> GSKKLINDVQDVLDEQLAGLAKAHPSLTLHQDPVYVTRADAPVAGKVALLSGGGSGHEPMHCGYIGQGMLSGACPGEIFTSPTPDKIFECAMQVDGGEGVLLIIKNYTGDILNFETATELLHDSGVKVTTVVIDDDVAVK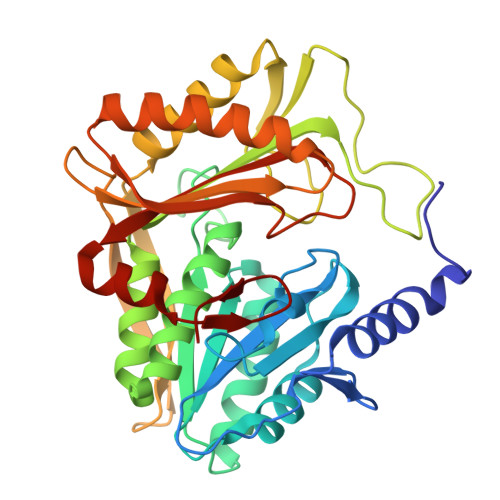DSLYTAGRRGVANTVLIEKLVGAAAERGDSLDACAELGRKLNNQGHSIGIALGACTVPAAGKPSFTLADNEMEFGVGIHGEPGIDRRPFSSLDQTVDEMFDTLLVNGSYHRTLRFWDYQQGSWQEEQQTKQPLQSGDRVIALVNNLGATPLSELYGVYNRLTTRCQQAGLTIERNLIGAYCTSLDMTGFSITLLKVDDETLALWDAPVHTPALNWGK>MTELIMESKHQLFKTETLTQNCNEILKRRRHVLVGISPFNSRFSEDYIHRLIAWAVREFQSVSVLLAGKEAANLLEALGTPHGKAERKVRKEVSRNRRFAEKALEAHGGNPED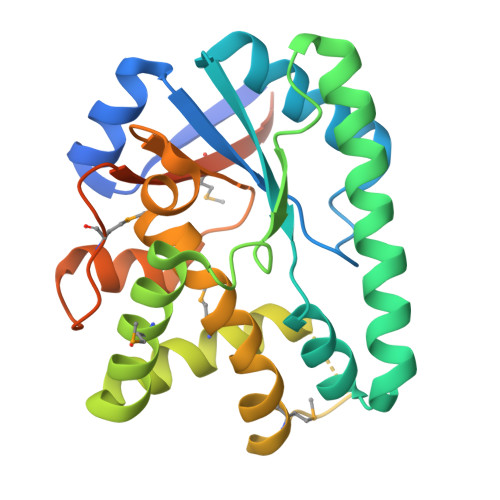IHTFSDFANQTAYRNLRMEVEAAFFDQTHFRNACLEMSHAAILGRARGTRMDVVEVSADMLELAVEYVIAELPFFIAAPDILGVEETLLAYHRPWKLGEQISRNEFAVKMRPNQGYLMVSEADERVESKSMQEERVLEHHHHHH[2x]>HMSNPLGELVKALEKLSFKPSDVRIYSLLLERGGMRVSEIARELDLSARFVRDRLKVLLKRGFV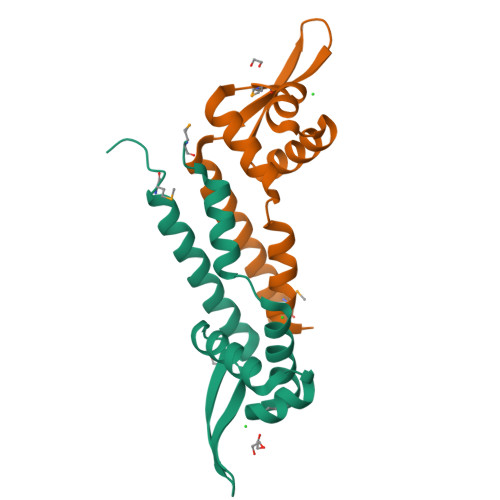RREIVEKGWVGYIYSAEKPEKVLKEFKSSILGEIERIEKMFTDGS[2x]>APQVVDKVAAVVNNGVVLESDVDGLMQSVKLNAAQARQQLPDDATLRHQIMERLIMDQIILQMGQKMGVKISDEQLDQAIANIAKQNNMTLDQMRSRLAYDGLNYNTYRNQIRKEMIISEVRNNEVRRRITILPQEVESLAQQVGNQNDASTELNLSHILIPLPENPTSDQVNEAESQARAIVDQARNGADFGKLAIAHSADQQALNGGQMGWGRIQELPGIFAQALSTAKKGDIVGPIRSGVGFHILKVNDLRGESKNISVTEVHARHILLKPSPIMTDEQARVKLEQIAADIKSGKTTFAAAAKEFSQDPGSANQGGDLGWATPDIFDPAFRDALTRLNKGQMSAPVHSSFGWHLIELL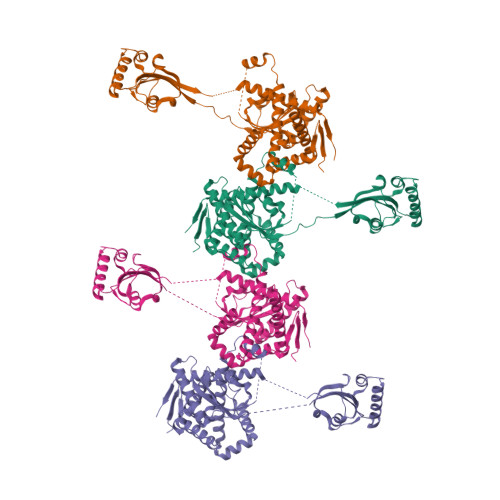DTRNVDKTDAAQKDRAYRMLMNRKFSEEAASWMQEQRASAYVKILSN[4x]methyl (2Z)-3-hydroxy-3-(3-hydroxyphenyl)prop-2-ene(dithioate) | C10 H10 O2 S2 | 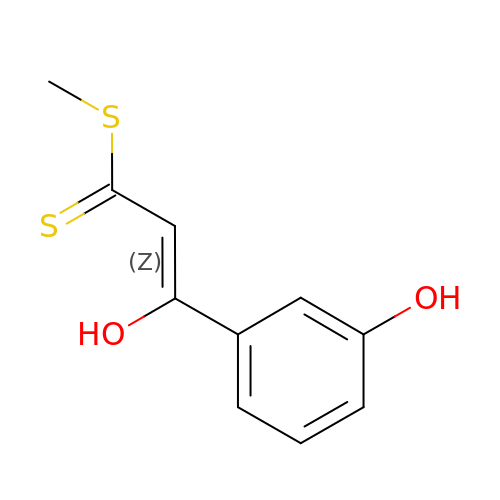MOMLKGNSDNGKFJ-TWGQIWQCSA-N>[2x]MRSRRVDVMDVMNRLILAMDLMNRDDALRVTGEVREYIDTVKIGYPLVLSEGMDIIAEFRKRFGCRIIADFKVADIPETNEKICRATF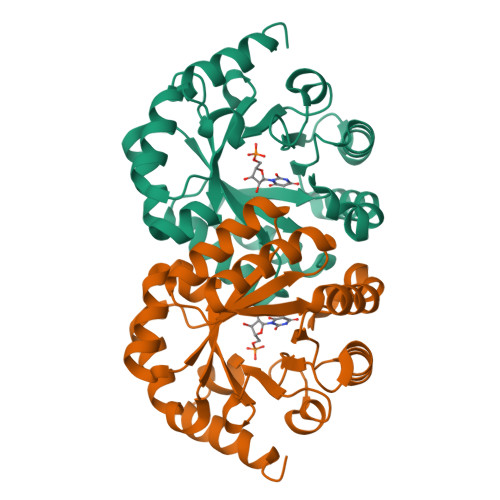KAGADAIIVHGFPGADSVRACLNVAEEMGREVFLLTEMSHPGAEMFIQGAADEIARMGVDLGVKNYVGPSTRPERLSRLREIIGQDSFLISPGVGAQGGDPGETLRFADAIIVGRSIYLADNPAAAAAGAIESIKDLLNP>[6x]MRGSHHHHHHGSMDKNIIIGAMTALITPFKNGKVDEQSYARLIKRQIENGIDAVVPVGTTGESATLTHEEHRTCIEIAVETCKGTKVKVLAGAG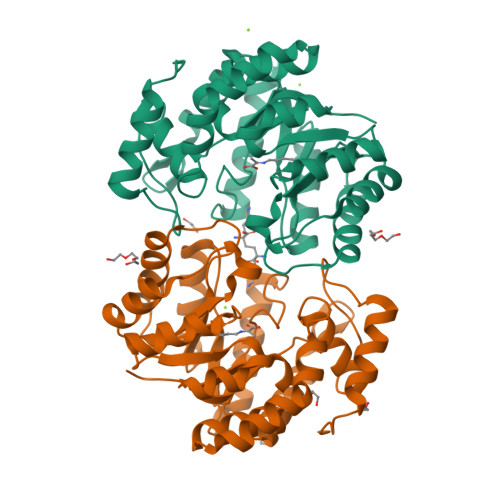SDATHEAVGLAKFAKEHGADGILSVAPYYNKPTQQGLYEHYKAIAQSVDIPVLLYNVPGRTGCEISTDTIIKLFRDCENIYGVKEASGNIDKCVDLLAHEPRMMLISGEDAINYPILSNGGKGVISVTSNLLPDMISALTHFALDENYKEAKKINDELYNINKILFCESNPIPIKTAMYLAGLIESLEFRLPLCSPSKENFAKIEEVMKKYKIKGF>[8x]M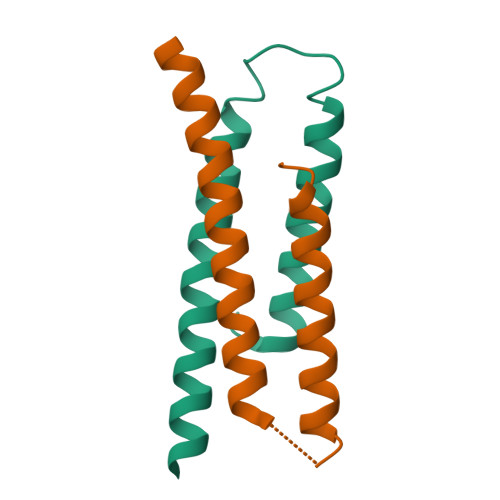TQLEEQLHNVETVRSITMQLEMALTKLKKDMMRGGDAKQYQVWQRESKALESAIAIIHYVAGDLK> MTSHSWLCDGRLLCLHDPSNKNNWKIFRECWKQGQPVLVSGVHKKLKSELWKPEAFSQEFGDQDVDLVNCRNCAIISDVKVRDFWDGFEIICKRLRSEDGQPMVLKLKDWPPGEDFRDMMPTRFEDLMENLPLPEYTKRDGRLNLASRLPSYFVRPDLGPKMYNAYGLITAEDRRVGTTNLHLDVSDAVNVMVYVGIPIGEGAHDEEVLKTIDEGDADEVTKQRIHDGKEKPGALWHIYAAKDAEKIRELLRKVGEEQGQENPPDHDPIHDQSWYLDQTLRKRLYEEYGVQGWAIVQFLGDAVFIPAGAPHQVHNLYSCIKVAEDFVSPE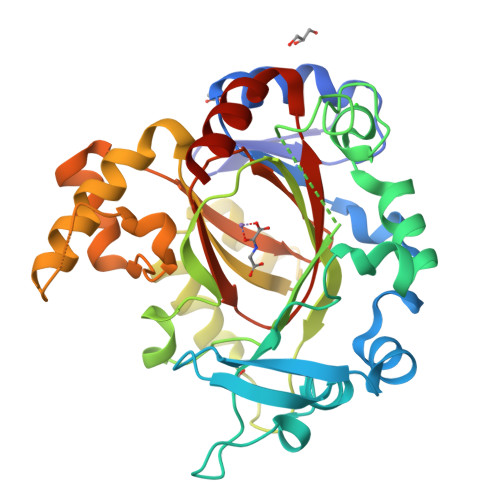HVKHCFRLTQEFAGNLYFQ>GMAGAIASRMSFSSLKRKQPKTFTVRIVTMDAEMEFNCEMKWKGKDLFDLVCRTLGLRETWFFGLQYTIKDTVAWLKMDKKVLDHDVSKEEPVTFHFLAKFYPENAEEELVQEITQHLFFLQVKKQILDEKIYCPPEASVLLASYAVQAKYGDYDPSVHKRGFLAQEELLPKRVINLYQMTPEMWEERITAWYAEHRGRARDEAEMEYLKIAQDLEMYGVNYFAIRNKKGTELLLGVDALGLHIYDPENRLTPKISFPWNEIRNISYSDKEFTIKPLDKKIDVFKFNSSKLRVNKLIL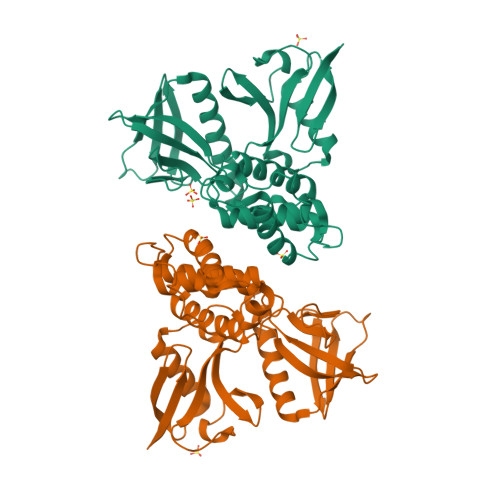QLCIGNHDLFMRRRKA[2x]>MHHHHHHHHHHGENLYFQGSDNIISFDHVTFTYPDSPRPALSDLSFAIERGSWTALIGHNGSGKSTVSKLINGLLAPDDLDKSSITVDGVKLGADTVWEVREKVGIVFQNPDNQFVGATVSDDVAFGLENRAVPRPEMLKIVAQAVADVGMADYADSEPSNLSGGQKQRVAIAGILAVKPQVIILDESTSMLDPEGKEQILDLVRKIKEDNNLTVISITHDLEEAAGADQVLVLDDGQLLDQGK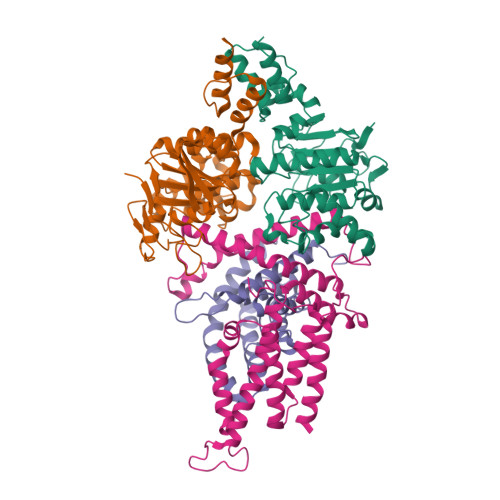PEEIFPKVEMLKRIGLDIPFVYRLKQLLKERGIVLPDEIDDDEKLVQSLWQLNSKM[2x];>MAIKFENVSYVYSPGSPLEAIGLDQLNFSLEEGKFIALVGHTGSGKSTLMQHFNALLKPTSGKIEIAGYTITPETGNKGLKDLRRKVSLAFQFSEAQLFENTVLKDVEYGPRNFGFSEDEAREAALKWLKKVGLKDDLIEHSPFDLSGGQMRRVALAGVLAYEPEIICLDEPAAGLDPMGRLEMMQLFKDYQAAGHTVILVTHNMDDVADYADDVLALEHGRLIKHASPKEVFKDSEWLQKHHLAEPRSARFAAKLEAAGLKLPGQPLTMPELADAIKQSLKGGEHE[2x];>MKSESKVSSKLELRELVLLAMVIAIKVILGQFKVGNATLQVGLGFIGSVMLGYLFGPWWGFAGGALSDLVSSVIFGNLGGFFIGFTLTAALGPMIYGFFLYKQPIQIWRVIASVICVTVICNIGLNTLWVSMMYGINFMVALSSRILKEMITPWIQMVAVWFILEGLSRVKLSRKFWSHPQFEK[2x];>[2x]MSKIIIGRYLPGTTFVYRVDPRAKLLTTFYFIIMIFLANNWVSYLVISIFGLAYVFATGLKARVFWDGVKPMIWMIVFTSLLQTFFMAGGKVYWHWWIFTLSSEGLINGLYVFIRFAMIILVSTVMTVTTKPLEIADAMEWMLTPLKLFKVNVGMISLVISIALRFVPTLFDQTVKIMNAQRSRGADFNDGGLVKRAKSVVPMLVPLFIDSLEVALDLSTAMESRGYKGSEGRTRYRILEWSKVDLIPVAYCLLLTILMITTRKH>GGRPAGPRVTVLVREFEAFDNAVPELVDSFLQQDPAQPVVVAADTLPYPPLALPRIPNVRLALLQPALDRPAAASRPETYVATEFVALVPDGARAEAPGLLERMVEALRAGSARLVAAPVATANPARCLALNVSLREWTARYGAAPAAPRCDALDGDAVVLLRARDLFNLSAPLARPVGTSLFLQTALRGWAVQLLDLTFAAARQPPLATAHARWKAEREGRARRAALLRALGIRLVSWEGGRLEWFGCNKETTRCFGTVVGDTPAYLYEERWTPPCCLRALRETARYVVGVLEAAGVRY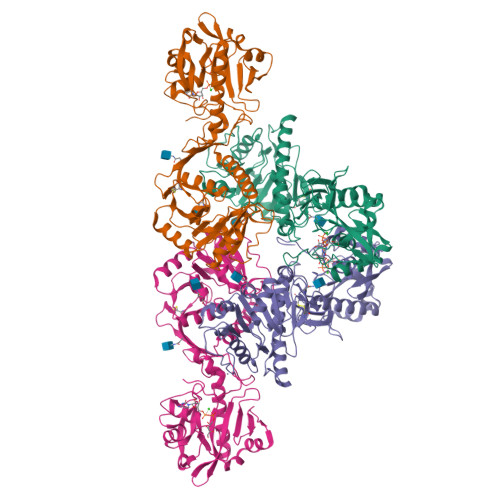WLEGGSLLGAARHGDIIPWDYDVDLGIYLEDVGNCEQLRGAEAGSVVDERGFVWEKAVEGDFFRVQYSESNHLHVDLWPFYPRNGVMTKDTWLDHRQDVEFPEHFLQPLVPLPFAGFVAQAPNNYRRFLELKFGPGVIENPQYPNPALLSLTGSG[4x]> YAE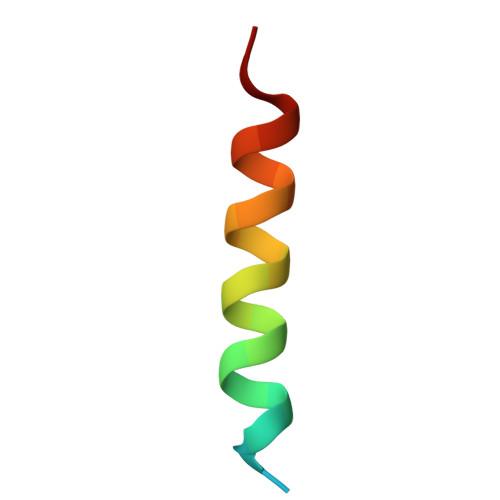NEKDSRRRQARLQKELAEAAKE> L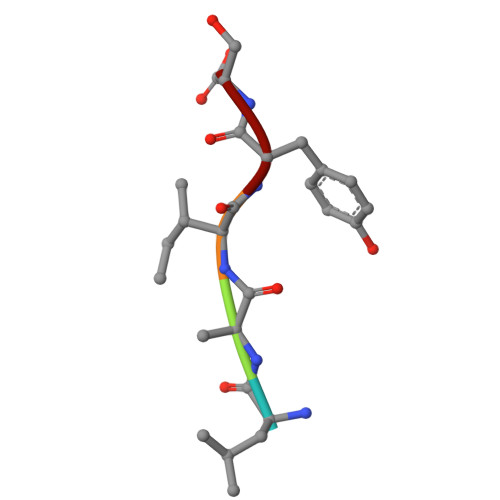AIYS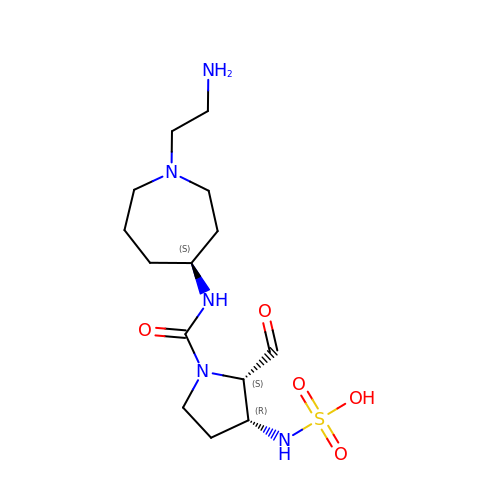[(2S,3R)-1-{[(4S)-1-(2-aminoethyl)azepan-4-yl]carbamoyl}-2-formylpyrrolidin-3-yl]sulfamic acid | C14 H27 N5 O5 S | FVHVSTMGNMLCNC-YNEHKIRRSA-N Sandercyanin (SFP) is a BV-binding lipocalin protein found in the skin mucus of the Canadian walleye, Stizostedion vitreum (formerly Sander vitreus). BV associates non-covalently to each SFP monomer in a ZZZssa conformation and is stabilized by aromatic stacking, hydrophobic interactions, and water-mediated H-bonding inside the lipocalin-like beta-barrel fold of SFP. The binding of BV induces tetramerization of SFP via interaction between amino acid residues from adjacent monomeric subunits. Using a combination of designed site-directed mutations, X-ray crystallography, UV/VIS, and resonance Raman spectroscopy, we have identified multiple conformations of BV that are stabilized in the binding pocket of SFP.

On excitation with 380 nm and 630 nm, Y142A showed a red-shifted fluorescence with maxima at 685 nm and a fluorescence quantum yield (0.004) equivalent to the monomeric SFP variants. We hypothesized that the mutation of the large Tyr into Ala created enough space for the D-ring to rotate in the tetrameric protein giving rise to dual peaks in the red region of the absorbance spectrum. To test this, we determined the crystal structure of the Y142A–BV complex at 2.65 Å (ESI Table S1†). However, to our surprise, the BV adopted the ZZZssa conformation in the crystal structure, with a water molecule accommodated in the position of the mutated side chain of Y142 (similar to the V71E structure). The similarity of BV conformation to the wild-type protein could not explain the observed differences in the absorption spectra. In contrast to the wild-type protein, BV bound to Y142A shows loss of fine structures of several RR bands in 532 nm excited spectra, specifically four bands at 1695, 1647, 1625, and 1596 cm−1 associated with D-ring in-plane stretching vibrations. Significant broadening of these RR bands strongly suggests the occurrence of multiple BV conformers bound to Y142A in the solution state. The increased stability provided to the ZZZssa conformation of BV by the residues of the neighboring subunit may be sufficient to shift the equilibrium towards this conformation in the high concentration of the protein in the crystals of Y142A. Hence, we conclude that both conformations of BV are possible in the Y142A variant in solution, even though only one is observed in the crystal structure.

>[2x]MFIKPGRCPKPAVQEDFDAARYLGVWYDIQRLPNKFQKGECATATYSLSPGVGFSVFNRERLANGTIKSVIGSAIAEDPCEPAKLQFFHENAAPVPYWVLSTDYDNYALVYSCINLGASHAAAASIVSRQPTLPEETIKKLQGTMSSFGVGVDTLLTTNQDAAYCSAMNQKLAAALEHHHHHH> MPSRTALSPGVLSPTRPVPNWIARPEYVGK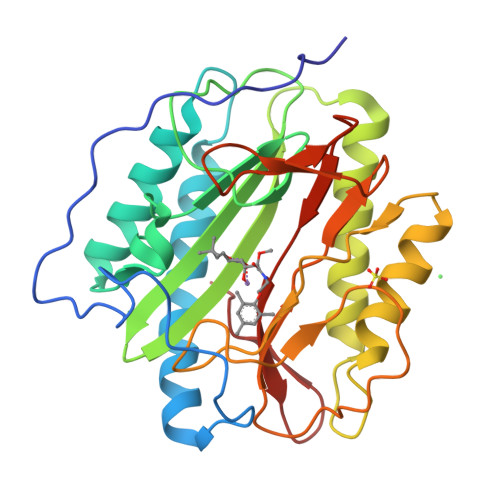PAAQEGSEPWVQTPEVIEKMRVAGRIAAGALAEAGKAVAPGVTTDELDRIAHEYLVDNGAYPSTLGYKGFPKSCCTSLNEVICHGIPDSTVITDGDIVNIDVTAYIGGVHGDTNATFPAGDVADEHRLLVDRTREATMRAINTVKPGRALSVIGRVIESYANRFGYNVVRDFTGHGIGTTFHNGLVVLHYDQPAVETIMQPGMTFTIEPMINLGALDYEIWDDGWTVVTKDRKWTAQFEHTLLVTDTGVEILTCL> KKKSPGEYVNI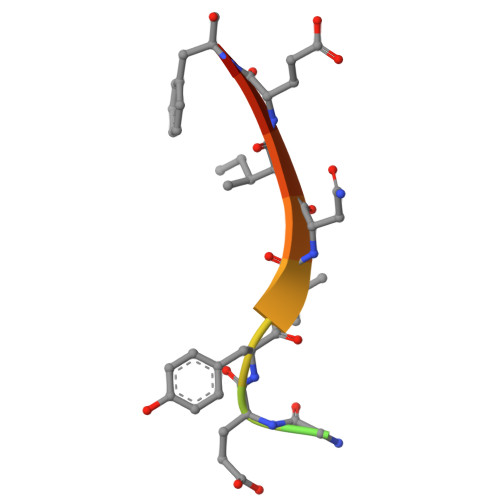EFG>MAYKYPSEKLFVEALKSKFAGLDLSDQKVKYVRAGYLQNARKREFQAAGERVAEQRGMQQYDVNVHLGGMTLGQRQLVPYKLSTRPDIVEGDDLHYVNNPAMQQMWDDMKRTIIVGMDLAHETLEKRLGKEVTPESIAGYMEAVNHTMPGAAIVQEHMVETHPGLVDDCYVKMFTGDDELADEIDSQYVININDLFDKEGQNEKLKAAIGKTTWQAVHIPTIVVRCCDGGNTSRWSAMQIGMSFIAAYNMCAGEAAVADLAFAAKHAAAVQMAEMLPARRARSPNEPGGLSFGYCADMVQTLRVKPEDPVWYTLEVVACGTMLYDQIWLGSYMSGGVGFTQYATAAYTNDVLDDFTYYGYDYALNKYGDDGTAPNDLATATDLATEVTLNGMECYEDYPTLLEDHFGGSQRAGILAAASACTTGIATGNSQVALSAWYMSMYVHKEGWGRLGFFGYDLQDQCGATNVCSYQGDEGCCLELRGANYPNYAMNVGHQGEYAGFTGSAHAGAHDAYCCNPLIKVCFADPSLVFDFSYIRKEYAKGAMRTFRPAGERSLVIPAGV[4x];>[4x]MADTIDLYDDRGKKLKGDVDLQAVSPLKNSAILSMVNTVKRTVAVNLAGIEKACKNASYGGQSRNIPGREVDIDPTAKADKIAARVKELIQVEKGDDTEVTVLGGGKFLRVAAPTRRIEAGAEYVAGMTCTAAALTEALREEYNLGLYDTPYVKNAVWGTYPQTMDMKGGNVLSVLSIPQNDEGLGFALRNIMANHLAMLSQRNAMNCAAISSILEHCGVFEMGQAIGLFERYQLLALAYQGLNANNMVYEMTKNNGKTGTIGTVVQETVGRALDDGVISVDKTMPSGYKVYKANDVCMWNAYCAAGTMAATMVNCGALRGAQAVSSTLLYFNDMIEKETSLPGCDWGRVEGTAVGFSFFSHSIYGGGGPGVFNGNHVVTRHSTGMAIPCVAVAVALDAGTQMFSPESTSAIVLDTFQDVPIMMNPLKEVAAAV;>MAYTPQYYPGSSHVAVNRRKHMSGDVEKLRTVSDDDLVAALGHRAPGADYPSTHPPLAEMGEPDCPVRQMVEPTPGAAAGDRVRYSQFTDSMYSAPSIPYFRSYYAAINFRGVDPGTLSGRQIVEARERDMEAQCKAAIESEMTCPALAGLRGCTVHGHSLRLAEDGMMFDMLQRTHIEGGNVIEDKDQVGVPIDRKVNLGKPMSDAEAKKRTTIYRTDGVKYRDEEEVLDHVHLVHHRRTMYGYRPETAAETAPGVGPVTYHTV[4x]

Here, we obtained the true atomic resolution structure of their methane-capturing system (Methyl-Coenzyme M Reductase, MCR), circumventing the isolation barrier by exploiting microbial enrichments of freshwater nitrate-reducing ANME-2d grown in bioreactors, and marine ANME-2c in syntrophy with bacterial partners. Methane capture, the first reaction in AOM, has been proposed to be carried out by the Methyl-Coenzyme M Reductase (MCR). In the proposed mechanism, the heterodisulfide, made of Coenzyme M (HS-CoM) and Coenzyme B (CoB-SH), would react with methane to generate methyl-S-CoM and free CoB-SH through a radical mechanism catalysed by the Ni-containing tetrapyrrole cofactor F43019,20. Despite their physiological differences, these ANMEs have extremely conserved MCR structures, similar to homologs from methanogenic Methanosarcinales, rather than the phylogenetically distant MCR of ANME-1 isolated from Black Sea mats.

The discovery of a gas channel in the ethane-capturing enzyme prompted us to investigate whether ANME-2 MCR possesses a similar access system for methane. Still, we performed krypton labelling on ANME-2c MCR crystals to verify the existence of an accessory tunnel via experimental means. Based on the anomalous signal of the dataset collected at the krypton K-edge, no signals were observed in the active site or tracking in a hydrophobic tunnel. Krypton atoms are rather positioned on the outer shell of the protein, trapped in hydrophobic pockets, as previously observed for the methanogenic enzyme from M. marburgensis. The absence of a dedicated gas tunnel connecting the active site to the solvent reinforces the proposed scenario that ethane-specialised homologues evolved this strategy by introducing loop extensions and dedicated PTMs. Labelling with gaseous krypton did not reveal any internal channels that would facilitate alkane diffusion to the active site, as observed in the ethane-specialised enzyme. Still, our structural insights showed that methane-oxidising MCRs do not contain gas tunnels that connect the solvent with the buried active site, in contrast to the ethane-activating enzyme. Our structural analysis suggests that methane first enters the catalytic site before the heterodisulfide closes the catalytic chamber.methyl beta-D-arabinopyranoside | 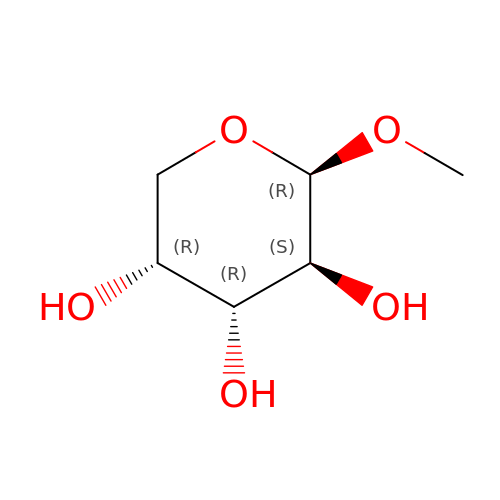C6 H12 O5 | ZBDGHWFPLXXWRD-ARQDHWQXSA-N> HHMSGLSDFF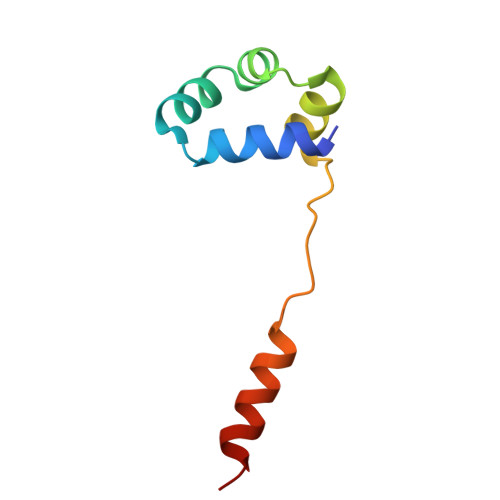TQLGQDAQLMEDYKQNPEAVMRAHGLTDEQINAVMTGDMEKLKTLSGDSSYQSYLVISHGNGD>GHMNDGNHYRTATSPNPSADTQPSDWAYIAEGGAHIVFSYQGQSKTYATRALRVRKPSATTESLAAAAANDVSGQWRRNILPKLVPRQLLTTSREVTLEEGWYKELLAMVDVVRPAQRKSAIDLAAKGDRRGVLLEDLTSNVDDDGAITVAIEIKPKWGFLPCAGHLQPPESVSIKSHVSRFRLHQHFRGRADDPPYDPLDLFSGDKMRMRTALDGLWTMWEISRGKSNNWKVFIGSKEISPDDLQRGLLPMGGDDLVTNITQLTLSALQTSSALPLLKNLQQNLDPIDISSLAALFQAEHPNSPIFDPDLIAEVSAVELNSFVDIYISDPQAGQRMDSWSLRE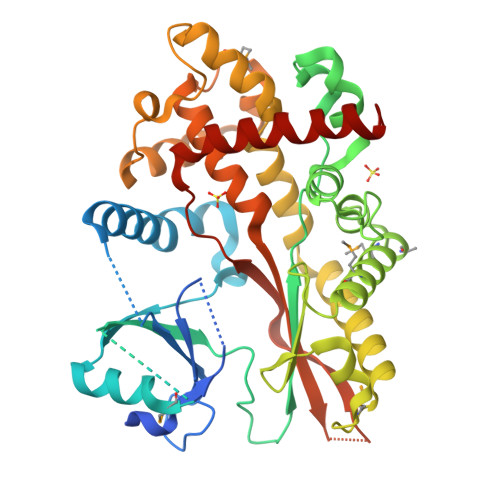RIIAYALSAIFKDCSLFVRGVLKHAEDGAWRLVSGGESVKVIDLDLKPVKNIQKWAETDEKVWKHWLKTKGTR[4x]Malate synthase, one of the two enzymes unique to the glyoxylate cycle, is found in all three domains of life, and is crucial to the utilization of two-carbon compounds for net biosynthetic pathways such as gluconeogenesis. The structures reported here for the glyoxylate and the pyruvate/acetyl-CoA complexes of Haloferax volcanii malate synthase represent the first examples of an H isoform member. The overall structure of hvMSH reveals that, like MSA and MSG, this halophilic isoform is based on a TIM barrel and indicates that deletion in hvMSH of an N-terminal domain distinguishes this isoform from those of MSA and MSG; and that the surface of the barrel normally buried by this domain and connecting loops is instead involved in trimeric and hexameric interfaces, suggesting a potential evolutionary coupling of the N-terminal deletion and oligomerization. Despite the sequence divergence and overall smaller size of hvMSH compared to MSA and MSG, the active site and catalytic mechanism are conserved in all three isoforms.

An atomic model was built manually into the experimental map, and was used for molecular replacement to solve the high-occupancy glyoxylate complex at 2.51 Å, and the pyruvate/acetyl-CoA complex. The high-occupancy glyoxylate complex was prepared by increasing the concentrations of MgCl2 from 13 mM to ~0.1 M and glyoxylate from 3 mM to ~0.1 M in mother liquor after crystal growth was complete and one week prior to data collection. The final model has a crystallographic Rfactor of 0.195 and an Rfree of 0.248, and is comprised of residues 5-283, 331-353, and 387-432, two glyoxylate molecules, one magnesium ion, three potassium ions, five chloride ions and 134 water molecules. One glyoxylate molecule is bound to the Mg2+ at the active site and the other is bound weakly in the position at which the acetyl-CoA thioester resides in the ternary complex (below). The structure is in good agreement with expected stereochemistry, with only one residue in the generously allowed region (Thr 276) and one residue in the disallowed region (Glu 24) of the Ramachandran plot. The enzyme also coordinates the magnesium ion with identical residues to those found in MSG and MSA: the side chains of Asp 192 and Glu 158 in hvMSH (Asp 455 and Glu 427 in ecMSG). Two water molecules complete the fifth and sixth positions in the magnesium coordination sphere with nearly perfect octahedral geometry as is seen in ecMSG. One notable difference in the active site between hvMSH and ecMSG is the conformation of the tryptophan residue adjacent to the aldehyde carbon of glyoxylate (Trp 257, and Trp 534 in hvMSH and ecMSG respectively). However, in the hvMSH complex the different rotomer positions the indole ring to interact more with its face than edge, with distances to the two closest carbons in the ring of 3.7 and 3.8 Å. The rotomer in the hvMSH structure is held in position by the side chain of Phe 14 which is packed against the opposite side of the indole ring.

> MTERRHDREFVRTFFTSPTAVEGEDDSAKMLRRAAGLRGMQAPDVWVPDNEDATAPSMRDEGAENIVEVISEQGAEFPGEIHPRMVWHRDSPETRYQGFQHMLDITDPERGAVEHIHGFVIPEVGGIDDWKKADEFFTIVEHEHGLDEGSLAMSVIIESGEAELAMGDLRDEMGKPTNNLERLFLLVDGEVDYTKDMRAMTPTGELPAWPELRHNTSRGASAAGCVAVDGPYDDIRDVEGYRERMTDNQAKGMLGIWSLTPGQVVEANTSPLPPKTGSWLLDADGEEVELASEDGVEAYDGDRLSLEATDGGYELRVGGDARELTADELREELLGLTSYVPSMDDIVDSMEEFEAAKEAGRGAIAMTQSATLRIGGTEIDIEKDRMWDEATYQAAMTPISLFQDVYENRPDQHEELEERYGAGVVERAMEVGL> GPEINKELNQVMEQLGDARIDRQESSRQQRKAEIMESIKRLYPGSVYGRLIDLCQPTQKKYQIAVTKVLGKNMDAIIVDSEKTGRDCIQYIKEQRGEPETFLPLDYLEVKPTDEKLRELKGAKLVIDVIRYEPPHIKKALQYACG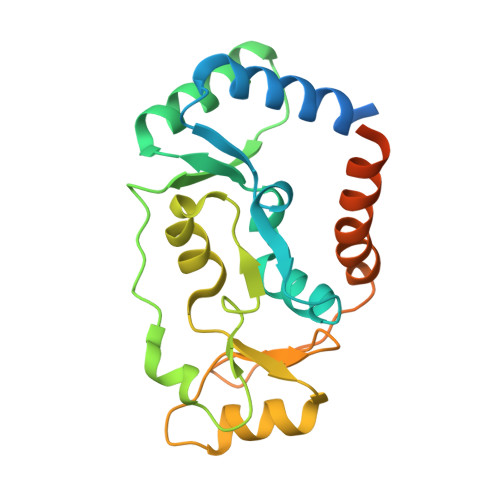NALVCDNVEDARRIAFGGHQRHKTVALDGTLFQKSGVISGGASDLKAKARRWDEKAVDKLKEKKERLTEELKEQMKAKRKEAELRQVQ>MDNSIHSTDGPDSVIPNSNPKKTVRQRVRLLARHLTTREGLIGDYDYGFLFRPELPFMKKDPRAPPFFGLNEKIPVLLAFILGLQHALAMLAGVVTPPLIISSSLSLPSDLQQYLVSTSLIVCGLLSMVQITRFHIYKTPYYIGSGVLSVMGVSFSIISVASGAFNQMYSNGFCQLDEAGNRLPCPEAYGALIGTSACCALVEILLAFVPPKVIQKIFPPIVTGPTVMLIGISLIGTGFKDWAGGSACMDDGMLCPSATAPRPLPWGSPEFIGLGFLVFVSIILCERFGAPIMKSCSVVIGLLVGCIVAAACGYFSHADIDAAPAASFIWVKTFPLSVYGPMVLPIIAVFIICACECIGDVTATCDVSRLEVRGGTFESRIQGAVLADGINSVVAALATMTPMTTFAQNNVVIALTRCANRWAGYCCCLILIVAGIFAKFAAAIVAIPNSVMGGMKTFLFASVVISGQAIVAKAPFTRRNRFILTASMALGYGATLVPTWFGNVFPQTENRDLEGFENAIELVLETGFAVTAFVAMLLNAIMPAEVEEIGAVTPMPVSAHDNRDGEAEYQSKQA[2x]

Nucleobase–ascorbate transporters (NATs), found in almost all species from bacteria and fungi to plants and mammals, are responsible for cellular uptake of essential metabolites. UapA from Aspergillus nidulans is specific for the purines xanthine and uric acid but does not transport hypoxanthine or adenine. The overall structure of UapA contains 14 transmembrane domains (TMs) organized into a 7+7 TM fold divided into a core (TMs 1–4 and 8–11) and a gate (TMs 5–7 and 12–14) domain, similar to UraA10. UapA forms a dimer with an extensive interface and a buried surface area of 6,000 Å2, involving TMs 12, 13 and 14 of the gate domain.

A thermostabilized construct of UapA with a single-residue substitution, G411V, and lacking the N-terminal 11 residues (UapA-G411VΔ1–11)17 was expressed in Saccharomyces cerevisiae as a green fluorescent protein (GFP) fusion protein. UapA-G411VΔ1–11 binds xanthine but is transport inactive. The structure in complex with xanthine was solved by single isomorphous replacement with anomalous scattering and refined at a resolution of 3.7 Å to an R-factor of 29.6% and Rfree of 32.7%. Density consistent with xanthine is visible in a clearly defined binding site approximately halfway across the membrane in a cleft formed by the half helices of TMs 3 and 10, similar to the uracil-binding site in UraA. The current structure confirms many of these earlier predictions, revealing xanthine is within hydrogen-bonding distance of the side chains of Gln408 (TM 10) and Glu356 (TM 8), the main chain nitrogen of Ala407 at the N terminus of TM 10 and the carbonyl oxygen of Val153 preceding TM 3, as well as the main chain nitrogen of Phe155 of TM 3. The phenyl rings of both Phe155 and Phe406 pack onto the xanthine. The residues directly interacting with the xanthine are all from the core domain and in the structure a detergent molecule packs over the xanthine separating it from TM 12 of the gate domain. The xanthine is fully accessible to the inward-facing side of the protein through this detergent-filled cavity. However, the UapA dimer structure reveals that this residue lies in close proximity to the xanthine-binding site, but of the opposite monomer.>FDSTDETPASYNLAVRRAAPAVVNVYNRGLNTNSHNQLEIRTLGSGVIMDQRGYIITNKHVINDADQIIVALQDGRVFEALLVGSDSLTDLAVLKINATGGLPTIPINARRVPHIGDVVLAIGNPYNLGQTITQGIISATGRIGLNPTGRQNFLQTDASINHGNSGGALVNSLGELMGINTLSFDKSNDGETPEGIGFAIPFQLATKIMDKLIRDGRVIRGYIGIGGREIAPLHAQGGGIDQLQGIVVNEVSPDGPAANAGIQVNDLI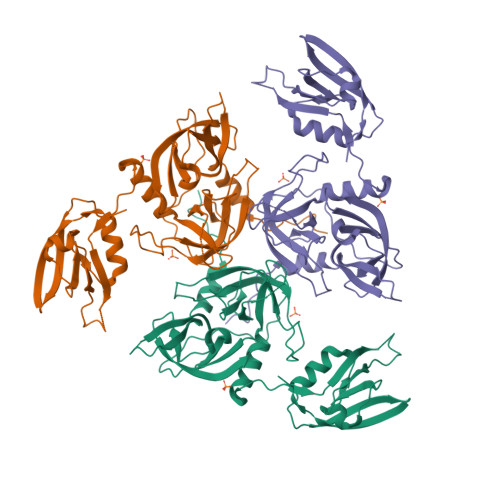ISVDNKPAISALETMDQVAEIRPGSVIPVVVMRDDKQLTLQVTIQEYPATN[2x]> PRLVGGDIPCSGRVEVQHGDTWGTVCDSDFSLEAASVLCRELQCGTVV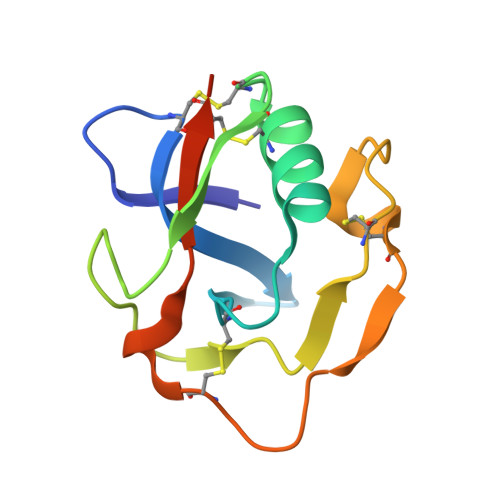SLLGGAHFGEGSGQIWAEEFQCEGHESHLSLCPVAPRPDGTCSHSRDVGVVCSVDHHHHHH>GCUUCGGCU[2x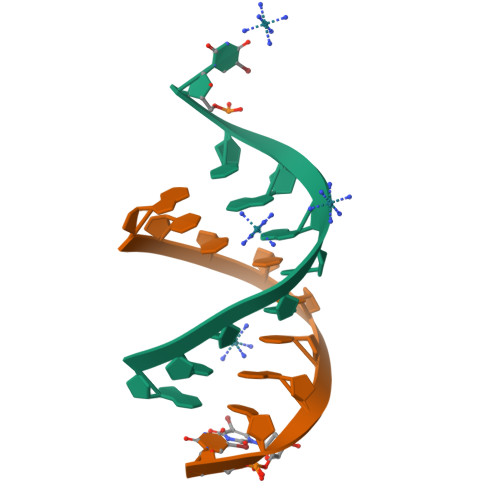]9-HYDROXYPROPYLADENINE, 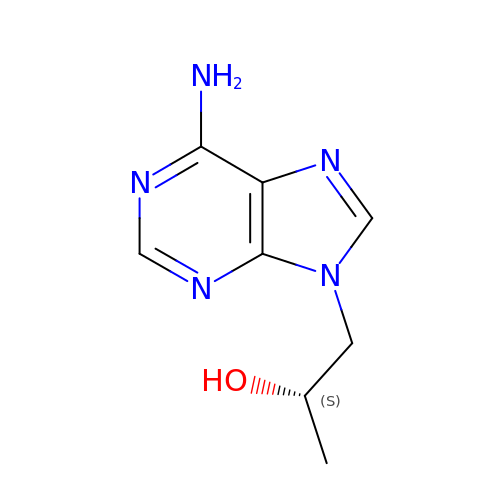S-ISOMER | C8 H11 N5 O | MJZYTEBKXLVLMY-YFKPBYRVSA-N>[3x]GSMSISISYSTTYSGWTVADYLADWSAYFGDVNHRPGQVV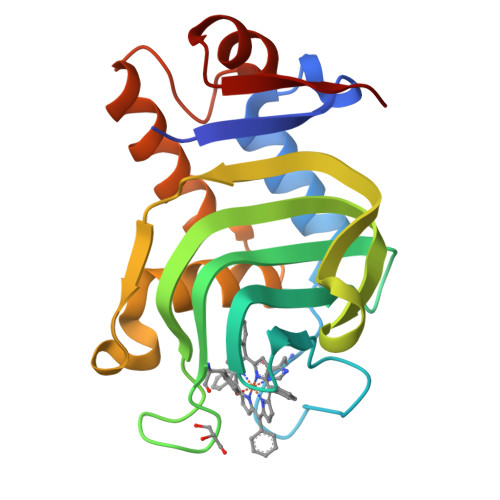DGSNTGGFNPGPFDGSQYALKSTASDAAFIAGGDLHYTLFSNPSHTAWGKLDSIALGDTLTGGASSGGYALDSQEVSFSNLGLDSPIAQGRDGTVHKVVYGLMSGDSSALQGQIDALLKAVDPSLSINSTFDQLAAAGVAHATPA> AVEPKEDTITVTAAPAPQESAWGPAATIAARQSATGTKTDTPIQKVPQSISVVTAEEMALHQPKSVKEALSYTPGVSVGTRGASNTYDHLIIRGFAAEGQSQNNYLNGLKLQGNFYNDAVIDPYMLERAEIMRGPVSVLYGKSSPGGLLNMVSKRPTTEPLKEVQFKAGTDSLFQTGFDFSDSLDDDGVYSYRLTGLARSANAQQKGSEEQRYAIAPAFTWRPDDKTNFTFLSYFQNEPETGYYGWLPKEGTVEPLPNGKRLPTDFNEGAKNNTYSRNEKMVGYSFDHEFNDTFTVRQNLRFAENKTSQNSVYGYGVCSDPANAYSKQCAALAPADKGHYLARKYVVDDEKLQNFSVDTQLQSKFATGDIDHTLLTGVDFMRMRNDINAWFGYDDSVPLLNLYNPVNTDFDFNAKDPANSGPYRILNKQKQTGVYVQDQAQWDKVLVTLGGRYDWADQESLNRVAGTTDKRDDKQFTWRGGVNYLFDNGVTPYFSYSESFEPSSQVGKDGNIFAPSKGKQYEVGVKYVPEDR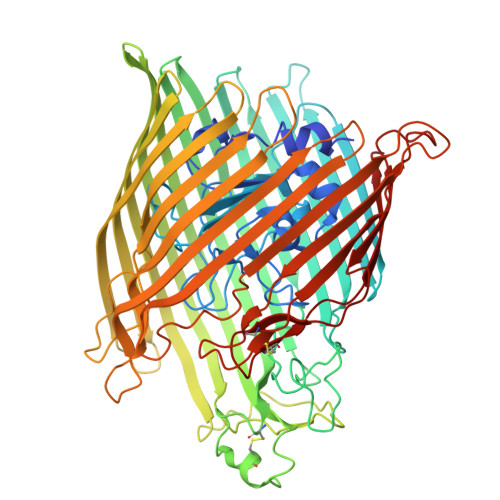PIVVTGAVYNLTKTNNLMADPEGSFFSVEGGEIRARGVEIEAKAALSASVNVVGSYTYTDAEYTTDTTYKGNTPAQVPKHMASLWADYTFFDGPLSGLTLGTGGRYTGSSYGDPANSFKVGSYTVVDALVRYDLARVGMAGSNVALHVNNLFDREYVASCFNTYGCFWGAERQVVATATFRF benzene-1,2,4-triol | C6 H6 O3 | 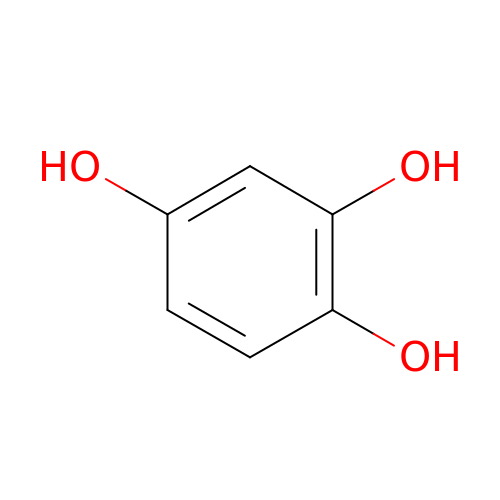GGNQRNBDZQJCCN-UHFFFAOYSA-N>[2x]TVKQNIIVTTEKEKRALTQEFVENMSPNDKVIMFVSQKHIADDLSSDFNIQGISAESLHGNSEQSDQERAVEDFKSGNIKILITTDIVSRGLDL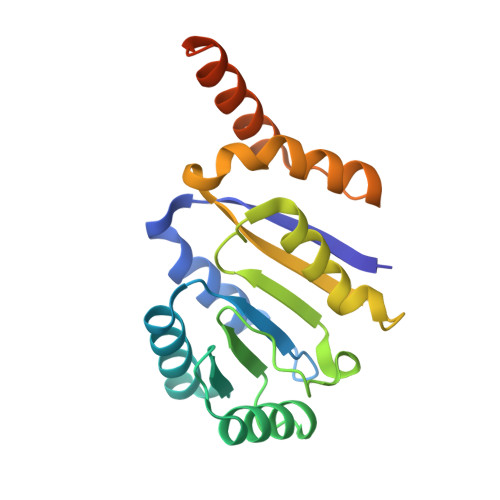NDVTHVYNYDFPRNIDVYVHRVGYIGRTGKTGTSVTLITQRDSKMAGELIKILDRANQSVPEDLVVMAEQYKLNQQKRHRETRSRKPGQRRKEFYFLS L-gamma-glutamyl-S-(2-{[4-(3-carboxypropyl)phenyl](2-chloroethyl)amino}ethyl)-L-cysteinylglycine 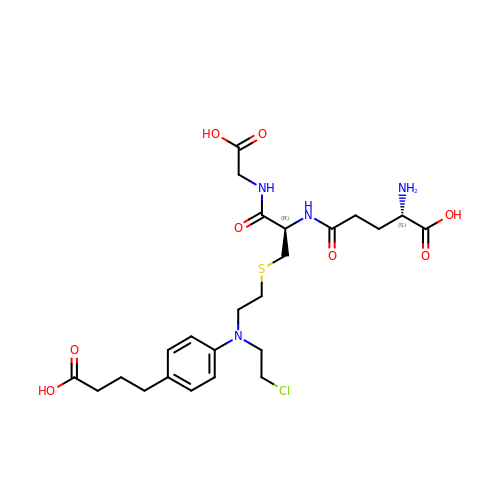| C24 H35 Cl N4 O8 S | BQVGPQFUMPRIMA-OALUTQOASA-N>SQLLNYIDGNFVTSASSFANINPVNGKLISDVFEADAKQVNEAVVAAQNALKGPWGKLSVQDRAALIHKIADGIQARFEEFVAAEVADTGRPVHQARTLDIPRAIANFRTFADLAKTSHTDLFEMSTSDGSGALNYTVRKPLGVIGVISPWNLPLLLFTWKVAPALACGNTVVAKPSEESPSSATLLAEVMHDAGVPPGVFNLIHGFGKDSAGEFLTQHPGISALTFTGESKTGSTIMKAVADGVKEVSFALGGKNAAVVFADADLDAAIEGVLRSSFTNSGQVCLCSERVYVHRSIFDEFVSGLKV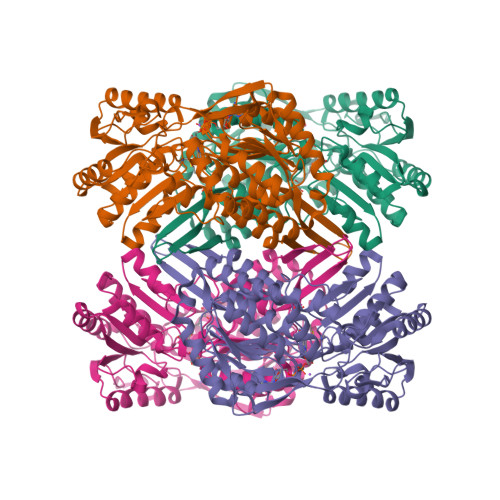EAERLVVGYPDQDGVNMGPLISHGHRDKVLSYYRLAVDEGATVVTGGGVPKFNDERDQGAYVQPTIWTGLSDKARCVTEEIFGPVCHISPFDDEDEVINRVNDSNYGLACAIWTTNLSRAHRVSRQIHVGLVWVNTWYLRDLRTPFGGVKLSGLGREGGRFSMDFYSDIANICIKI[4x]>[6x]MTPHINAKIGDFYPQCLLCGDPLRVSYIAKKFLQDAKEITNVRNMLGFSGKYKGKGISLMGHGMGIASCTIYVTELIKTYQ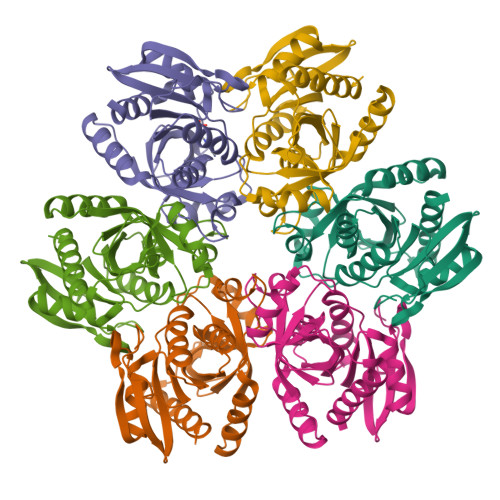VKELLRIGTCGAISPKVGLKDIIMATGASTDSKTNRVRFLNHDLSATPDFELSLRAYQTAKRLGIDLKIGNVFSSDFFYSFETHAFDLMAQYNHLAIEMEAAGLYATAMELNAKALCLCSVSDHLITKEALSPKERIESFDNMIILALEMMS>[4x]MRLPDPYTNPEYPGLGFESVNLVDNDPMIRDELP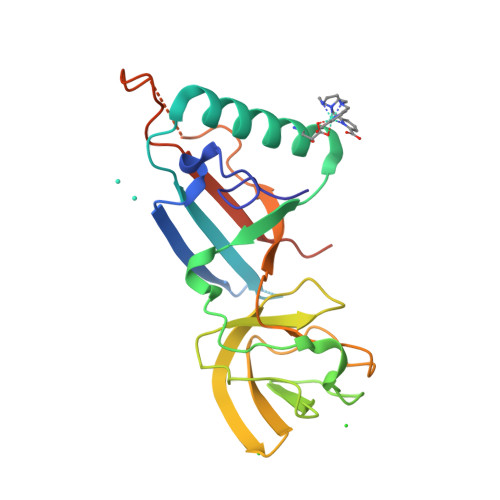NGKVKEVKISAQYWGINISYPELFPDEYAFLDSRLLEYKRTGDYLDVLLPQYEAFRVRGDTKSVTIPAGQKGSQIILNTNGTLTGQPKAGDLFKLSTHPKVYKITNFSSSGNVWNISLYPDLFITTTGSEKPVFNGILFRTKLMNGDSFGSTLNNNGTYSGISLSLRESLENLYFQGHHHHHH(1R,3R,7E,17beta)-17-[(1R)-6,6,6-trifluoro-5-hydroxy-1-(4-hydroxy-4-methylpentyl)-5-(trifluoromethyl)hex-3-yn-1-yl]-9,10-secoestra-5,7-diene-1,3-diol 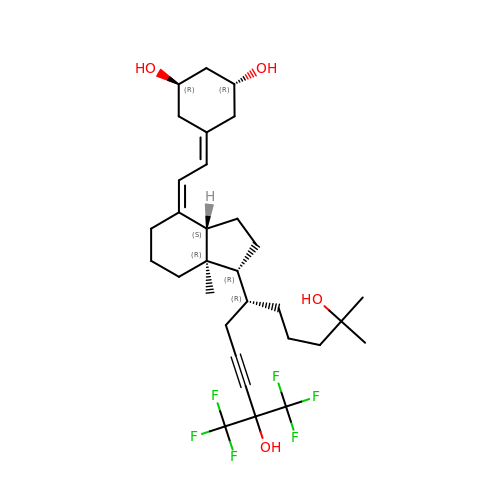| C31 H44 F6 O4 | RAYDHJNMFBHXHA-DUSBBPLISA-N>[2x]MDTFVSRLPVSQPQEHPMACCCKDREKKTAESGSICEARIDFVFPEVKFPSKKVYLA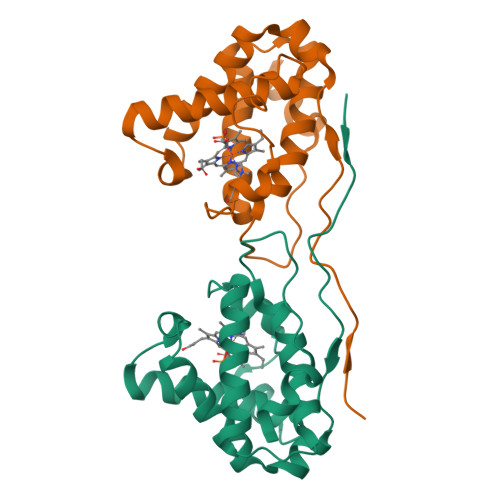AGEELLRKLVEVHHENLMKSKIHYLFPTSHEQLRSLVKRSADFVVEMCGGPPYYTLTRGEPKMRARHFSVTIDEKAREIWLACYKHALKDVHFPLSVLEEFWQWIESFSIRMINRRTTLEPPRRVPYSEIQDFFVS Mechanosensitive (MS) ion channels are a ubiquitous type of molecular force sensor sensing forces from the surrounding bilayer. Here we determine the structures of plant and mammalian OSCA/TMEM63 proteins, allowing us to identify essential elements for mechanotransduction and propose roles for putative bound lipids in OSCA/TMEM63 mechanosensation. Briefly, the central cavity created by the dimer interface couples each subunit and modulates dimeric OSCA/TMEM63 channel mechanosensitivity through the modulating lipids while the cytosolic side of the pore is gated by a plug lipid that prevents the ion permeation.

Inspired by the observation of the extended state of AtOSCA1.1 channels in the nanodisc, we attempted to solve the high-resolution structure of another member of the OSCA/TMEM63 channel family, the higher pressure activated mechanosensitive atOSCA3.1 channel which exhibits a half activation pressure threshold that is much higher than that of AtOSCA1.1. Our high-resolution cryo-EM data obtained in a detergent environment contain two conformations of AtOSCA3.1 channels. One is identical to our previously low-resolution model of AtOSCA3.113, which we call an extended state. The other is a more compact contracted state. We analyzed each monomer of AtOSCA3.1 in the two states and found that the single monomer of the contracted state superimposes with the extended state. Therefore, the major conformational change occurs in the central cavity. In the contracted state, each subunit of the M5 and M6 linker forms another dimer interface through an L487 interaction. Therefore, the area of the central cavity is reduced compared to the extended state. The disruption of the M5 and M6 linker interaction and extension of the central cavity is likely an energy barrier for channel transition to the extended state and then opening of the channel. Furthermore, the dimer interface of the AtOSCA3.1 in the contracted state was ‘locked’ by the interaction between each single subunit through the M5 and M6 linker, presumably providing an additional energy barrier to overcome during activation.

>[2x]MEFGSFLVSLGTSFVIFVILMLLFTWLSRKSGNAPIYYPNRILKGLEPWEGTSLTRNPFAWMREALTSSEQDVVNLSGVDTAVHFVFLSTVLGIFACSSLLLLPTLLPLAATDNNIKNTKNATDTTSKGTFSQLDNLSMANITKKSSRLWAFLGAVYWISLVTYFFLWKAYKHVSSLRAQALMSADVKPEQFAILVRDMPAPPDGQTQKEFIDSYFREIYPETFYRSLVATENSKVNKIWEKLEGYKKKLARAEAILAATNNRPTNKTGFCGLVGKQVDSIEYYTELINESVAKLETEQKAVLAEKQQTAAVVFFTTRVAAASAAQSLHCQMVDKWTVTEAPEPRQLLWQNLNIKLFSRIIRQYFIYFFVAVTILFYMIPIAFVSAITTLKNLQRIIPFIKPVVEITAIRTVLESFLPQIALIVFLAMLPKLLLFLSKAEGIPSQSHAIRAASGKYFYFSVFNVFIGVTLAGTLFNTVKDIAKNPKLDMIINLLATSLPKSATFFLTYVALKFFIGYGLELSRIIPLIIFHLKKKYLCKTEAEVKEAWYPGDLSYATRVPGDMLILTITFCYSVIAPLILIFGITYFGLGWLVLRNQALKVYVPSYESYGRMWPHIHQRILAALFLFQVVMFGYLGAKTFFYTALVIPLIITSLIFGYVCRQKFYGGFEHTALEVACRELKQSPDLEEIFRAYIPHSLSSHKPEEHEFKGAMSRYQDFNAIAGV>[2x]GRSGVIGLAVPELGQAFFAQLADEVIRVAAEQDLVVLVEQTGGLRERELEALRNPRLSLTDGLLLAPLGLTQDDVLPDPAGRPLVVLGEPLFPGPVDHVTMQHEAAARAATEHLLGLGRRRVMLLGAHATERTGVAALRYAGYREALTAAGLAVDDDLVVPVETWDRSSGAEAMARVLDAGVRMDAVFAMNDDLALGALRSLQERGVAVPGDVALMG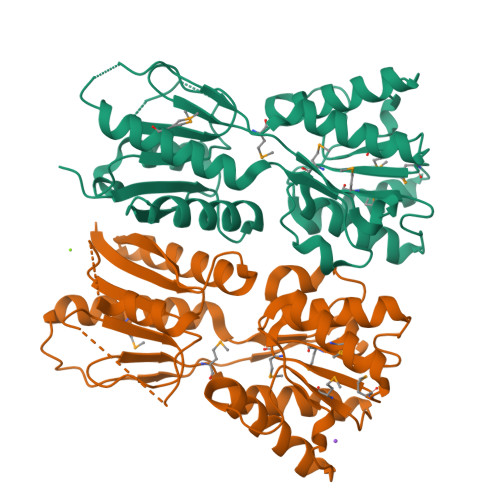FDDVADGRYTYPSLTTVEPGRHDIARAAVTMLSERIADAGTGAIEPRLTAPEFRLVVRESTGG> E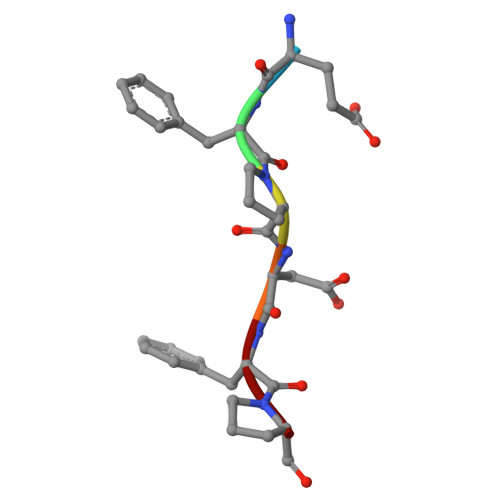FPDFP> ANVWGVRLADSLSSPTIETRTRQYTLHDLCSDLDANPGREPWKPLRNQRTNNIVAVQLFRPLQGLVLDTQLYGFPGAFDDWERFMREKLRVLKYEVLRIYPISNYSNEHVNVFVANALVGAFLSNQAFYDLLPLLIINDTMIGDLLGTGASLSQFFQSHGDVLEVAAGRKYLQMENYSNDDDDPPLFAKDLSDYAKAFYSDTYEVLDRFFWTHDSSAGVLVHYDKPTNGHHYLLGTLTQMVSAPPYIINATDAMLLESCLEQFSANVRARPAQPVTRLDQCYHLRWGAQYVGEDSLTYRLGVLSLLATNGYQLARPIPRQLTNRWLSSFVSQIMSDGVNETPLWPQERYVQIAYDSPSVVDGATQYGYVRKNQLRLGMRISALQSLSDTPSPVQWLPQYTIDQAAMDEGDLMVSRLTQLPLRPDYGNIWVGDALSYYVDYNRSHRVVLSSELPQLPDTYFDGDEQYGRSLFSLARKIGDRSLVKDTAVLKHAY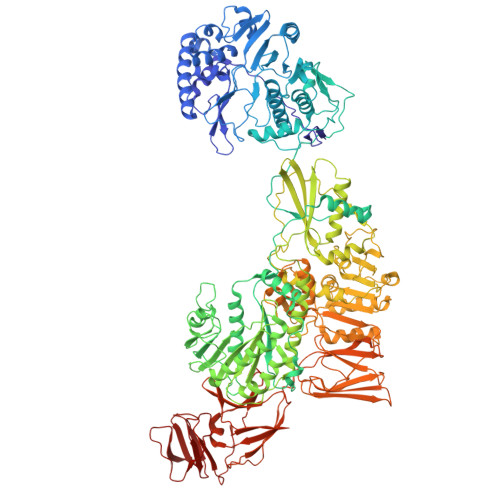QAIDPNTGKEYLRSRQSVAYFGASAGHSGADQPLVIEPWIQGKISGVPPPSSVRQFGYDVARGAIVDLARPFPSGDYQFVYSDVDQVVDGHDDLSISSGLVESLLSSCMHATAPGGSFVVKINFPTRPVWHYIEQKILPNITSYMLIKPFVTNNVELFFVAFGVHQHSSLTWTSGVYFFLVDHFYRYETLSTISRQLPSFGYVDDGSSVTGIETISIENPGFSNMTQAARIGISGLCANVGNARKSIAIYESHGARVLTITSRRSPASARRKSRLRYLPLIDPRSLEVQARTILPADPVLFENVSGASPHVCLTMMYNFEVSSAVYDGDVVLDLGTGPEAKILELIPATSPVTCVDIRPTAQPSGCWNVRTTFLELDYLSDGWITGVRGDIVTCMLSLGAAAAGKSMTFDAAFQQLIKVLSKSTANVVLVQVNCPTDVVRSIKGYLEIDSTNKRYRFPKFGRDEPYSDMDALEKICRTAWPNCSITWVPLSYDLRWTRLALLESTTLSSASIRIAELMYKYMPIMRIDIHGLPMEKRGNFIVGQNCSLVIPGFNAQDVFNCYFNSALAFSTEDVNAAMIPQVSAQFDATKGEWTLDMVFSDAGIYTMQALVGSNANPVSLGSFVVDSPDVDITDAWPAQLDFTIAGTDVDITVNPYYRLMTFVRIDGQWQIANPDKFQFFSSASGTLVMNVKLDIADKYLLYYIRDVQSRDVGFYIQHPLQLLNTITLPTNEDLFLSAPDMREWAVKESGNTICILNSQGFVLPQDWDVLTDTISWSPSIPTYIVPPGDYTLTPL2,2'-Anhydro-(1-beta-D-ribofuranosyl)uracil 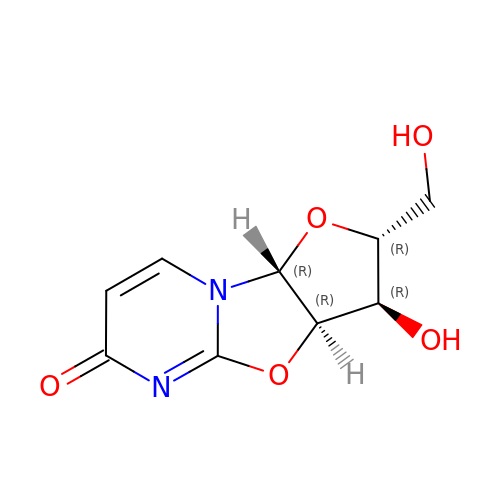| C9 H10 N2 O5 | UUGITDASWNOAGG-XVFCMESISA-N>ADTIDATTRLVLRSISERAAVDRISESFGRSAQVMHDPFGGQPFPAANSPWAPVLAGQGGPFDAETRRVSWETLVAHGPSLYRTFAGNPRAASTAKAMRDCVLRQENFIEALASADETLAWCKMCIHHNLPLRPQDPIIGTAAAVLDNLATRLRPFLQCYLKARGLCGLDELCSRRRLADIKDIASFVFVILARLANRVERGVAEIDYATLGVGVGEKMHFYLPGACMAGLIEILDTHRQECSSRVCELTASHIVAPPYV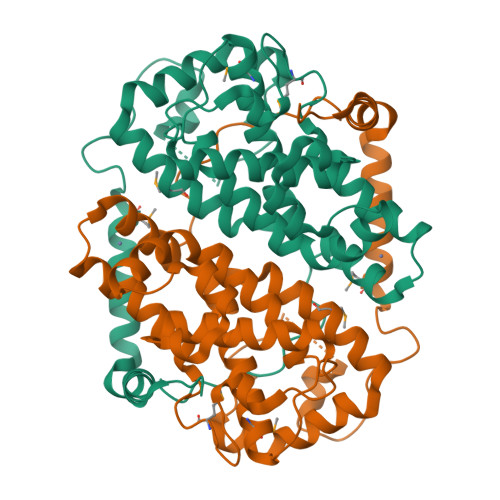HGKYFYCNSLF[3x]> MSYQNLVSEAGLTQKLLIHGDKELFQHELKTIFARNWLFLTHDSLIPSPGDYVKAKMGVDEVIVSRQNDGSVRAFLNVCRHRGKTLVHAEAGNAKGFVCGYHGWGYGSNGELQSVPFEKELYGDAIKKKCLGLKEVPRIESFHGFIYGCFDAEAPPLIDYLGDAAWYLEPTFKYSGGLELVGPPGKVVVKANWKSFAENFVGDGYHVGWTHAAALRAGQSVFSSIAGNAKLPPEGAGLQMTSKYGSGMGVFWGYYSGNFSADMIPDLMAFGAAKQEKLAKEIGDVRARIYRSFLNGTIFPNNSFLTGSAAFRVWNPIDENTTEVWTYAFVEKDMPEDLKRRVADAVQRSIGPAGFWESDDNENMETMSQNGKKYQSSNIDQIASLGFGKDVYGDECYPGVVGKSAIGETSYRGFYRAYQAHISSSNWAEFENASRNWHIEHTKTTDR;> MMINTQEDKLVSAHDAEEFHRFFVGHDSDLQQEVTTLLTREAHLLDIQAYKAWLEHFVAPEIKYQVISRELRSTSERRYQLNDAVNLYNENYQQLKVRVEHQMDPQNWANNPKIRFTRFVTNVTAAKDKSAPEILHVRSNLILHRARRENQVDVFYATREDKWKRIEGGGIKLVERFVDYPERIP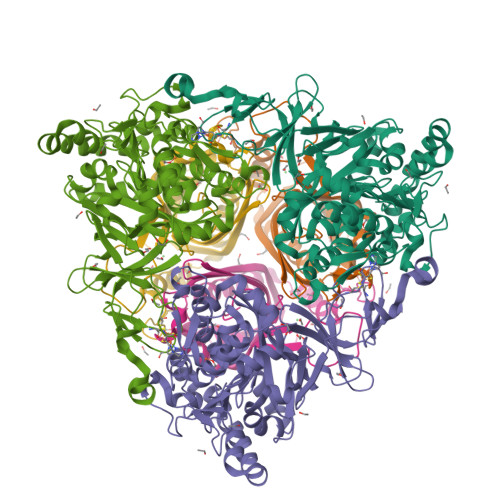QTHNLLVFL>GPLGSKYDFSCELYRMSTYSTFPAGVPVSERSLARAGFYYTGVNDKVKCFCC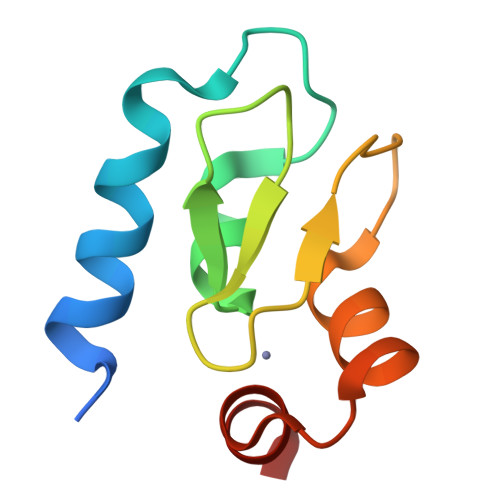GLMLDNWKLGDSPIQKHKQLYPSCSFIQNLVSA[2x]>[4x]MVKTEPLQITTELPGRTSAYRIAEVRPQVSGIILKRNFKEGSDIEAGVSLYQIDPATYQATYDSAKGDLAKAQAAANIAQLTVNRYQKLLGTQYISKQEYDQALADAQQANAAVTAAKAAVETARINLAYTKVTSPISGRIGKSNVTEGALVQNGQATALATVQQLDP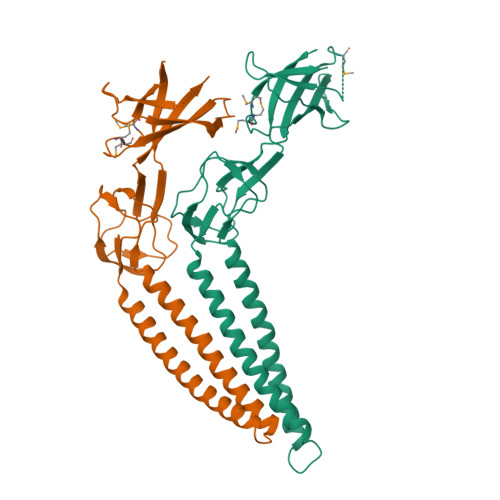IYVDVTQSSNDMMRLKQELANGTLKQENGKAKVSLITSDGIKFPQDGTLEFSDVTVDQTTGSITLRAIFPNPDHTMMPGMFVRARLEEGLNPNAILVPQQGLEHHHHHH> HSKCYAGATFATEAPQVTTL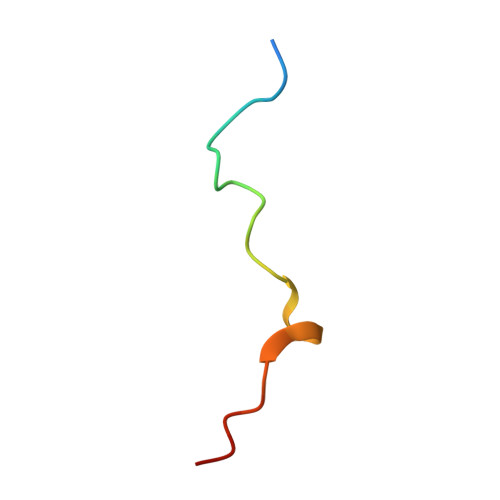PKPSFV>[2x]MVPISPIETVPVKLKPGMDGPKVKQWPLTEEKIKALVEICTEMEKEGKISKIGPENPYNTPVFAIKKKDSTKWRKLVDFRELNKRTQDFWEVQLGIPHPAGLKQKKSVTVLDVGDAYFSVPLDKDFRKYTAFTIPSINNETPGIRYQYNVLPMGWKGSPAIFQSSMTKILEPFRKQNPDIVIYQYMDDLYVG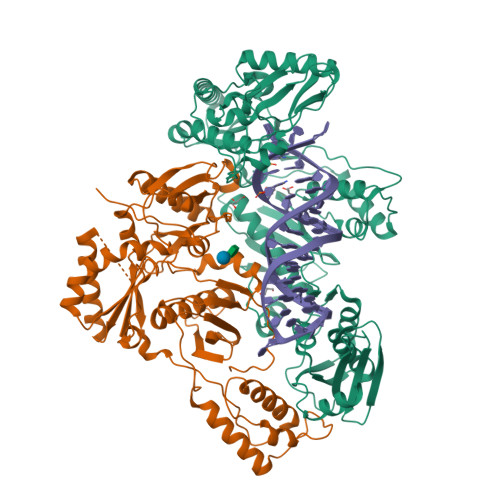SDLEIGQHRTKIEELRQHLLRWGFTTPDKKHQKEPPFLWMGYELHPDKWTVQPIVLPEKDSWTVNDIQKLVGKLNWASQIYAGIKVRQLSKLLRGTKALTEVVPLTEEAELELAENREILKEPVHGVYYDPSKDLIAEIQKQGQGQWTYQIYQEPFKNLKTGKYARMKGAHTNDVKQLTEAVQKIATESIVIWGKTPKFKLPIQKETWEAWWTEYWQATWIPEWEFVNTPPLVKLWYQLEKEPIIGAETFYVDGAANRETKLGKAGYVTDRGRQKVVPLTDTTNQKTELQAIHLALQDSGLEVNIVTDSQYALGIIQAQPDKSESELVSQIIEQLIKKEKVYLAWVPAHKGIGGNEQVDKLVSAG;>MAHHHHHHALEVLFQGPISPIETVPVKLKPGMDGPKVKQWPLTEEKIKALVEICTEMEKEGKISKIGPENPYNTPVFAIKKKDSTKWRKLVDFRELNKRTQDFWEVQLGIPHPAGLKQKKSVTVLDVGDAYFSVPLDKDFRKYTAFTIPSINNETPGIRYQYNVLPQGWKGSPAIFQSSMTKILEPFRKQNPDIVIYQYMDDLYVGSDLEIGQHRTKIEELRQHLLRWGFTTPDKKHQKEPPFLWMGYELHPDKWTVQPIVLPEKDSWTVNDIQKLVGKLNWASQIYAGIKVRQLSKLLRGTKALTEVVPLTEEAELELAENREILKEPVHGVYYDPSKDLIAEIQKQGQGQWTYQIYQEPFKNLKTGKYARMKGAHTNDVKQLTEAVQKIATESIVIWGKTPKFKLPIQKETWEAWWTEYWQATWIPEWEFVNTPPLVKLWYQ[2x]>[2x]MLSNLKTGNNILGLPEFELNGCRFLYKKGIEKTIITFSAFPPKDIAQKYNYIKDFLSSNYTFLAFLDTKYPEDDARGTYYITNELDNGYLQTIHCIIQLLSNTNQEDTYLLGSSKGGVGALLLGLTYNYPNIIINAPQAKLADYIKTRSKTILSYMLGTSKRF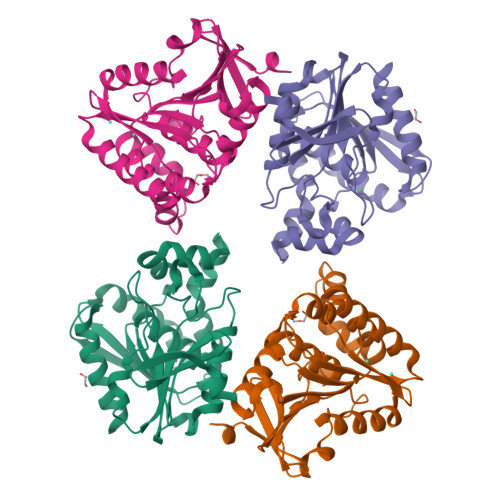QDINYDYINDFLLSKIKTCDSSLKWNIHITCGKDDSYHLNELEILKNEFNIKAITIKTKLISGGHDNEAIAHYREYFKTIIQNILEHHHHHH>RFYVKDHRNKAMINLHIQKDNPKIVHAFDMEDLAAKAVYCRCWRSKKFPFCDGAHTKHNEETGDNVG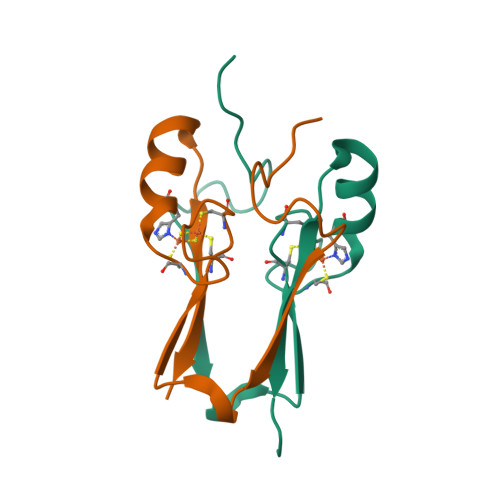PLIIKKKET[2x]> GSHMEEAKGPVKHVLLASFKDGVSPEKIEELIKGYANLVNLIEPMKAFHWGKDVSIENLHQGYTHIFESTFESKEAVAEY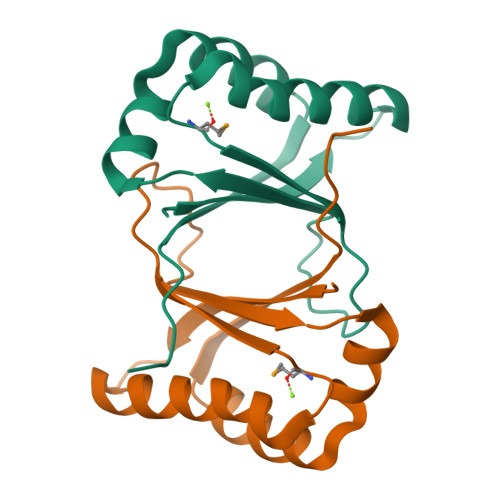IAHPAHVEFATIFLGSLDKVLVIDYKPTSVSL> MQEPLAAGAVILRRFAFNAAEQLIRDINDVASQSPFRQMVTPGGYTMSVAMTNCGHLGWTTHRQGYLYSPIDPQTN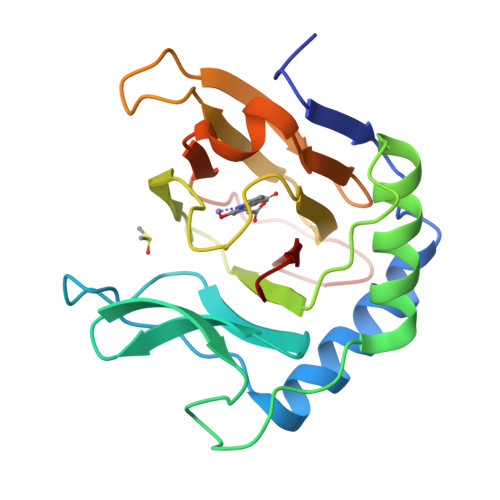KPWPAMPQSFHNLCQRAATAAGYPDFQPDACLINRYAPGAKLSLHQDKDEPDLRAPIVSVSLGLPAIFQFGGLKRNDPLKRLLLEHGDVVVWGGESRLFYHGIQPLKAGFHPLTIDCRYNLTFRQAGKKE> MSSLSRELVFLILQFLDEEKFKETVHKLEQESGFFFNMKYFEEKVHAGEWDEVEKYLSGFTKVDDNRYSMKIFFEIRKQKYLEALDRHDRAKAVDILVKDLKVFSTFNEELYKEITQLLTLENFRENEQLSKYGDTKSARSIMLIELKKLIEANPLFRE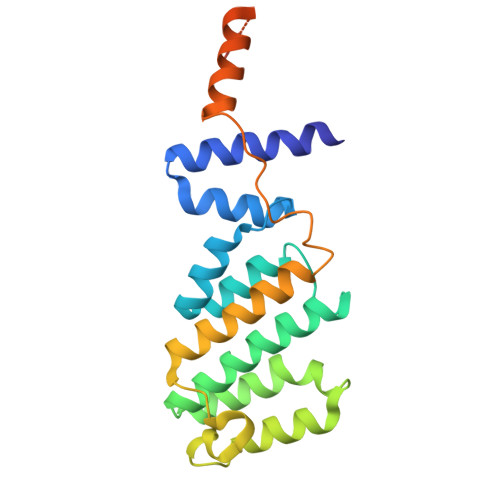KLVFPTLKASRLRTLINQSANWQHQLCKNPRPNPDAKTLFTDHTCTPPNG>GAMGQTTFTEL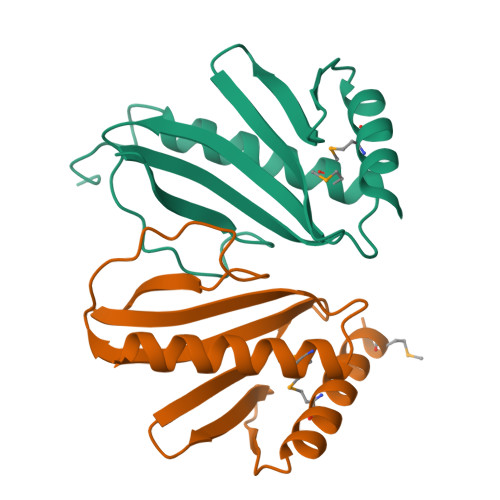MQQLFLKLGLNHQVNENDVYTFEVDGHIQVLIACYHQQWVQLFSELGADLPTNDNLFGEHWPAHVQGRLDGKSILWSQQSLVGLDIDEMQAWLERFIDDIEQRKEPQNTKFQPN[2x]> GHMLVMRPAQAADLPQVQRLAADSPVGVTSLPDDAERLRDKILA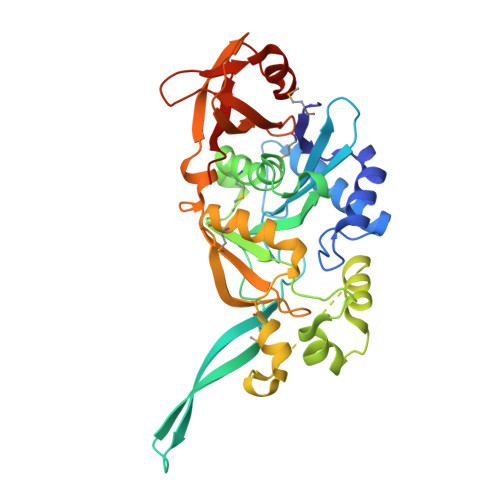SEASFAAEVSYNGEESYFFVLEDSASGELVGCSAIVASAGFSEPFYSFRNETFVHASRSLSIHNKIHVLSLCHDLTGNSLLTSFYVQRDLVQSVYAELNSRGRLLFMASHPERFADAVVVEIVGYSDEQGESPFWNAVGRNFFDLNYIEAEKLSGLKSRTFLAELMPHYPIYVPLLPDAAQESMGQVHPRAQITFDILMREGFETDNYIDIFDGGPTLHARTSGIRSIAQSRVVPVKIGEAPKSGRPYLVTNGQLQDFRAVVLDLDWAPGKPVALSVEAAEALGVGEGASVRLVAVGS>[2x]MSQEQLVAVNELNENLGKVLIKIARDSIANKLGILKINLEDYLSSLNDPI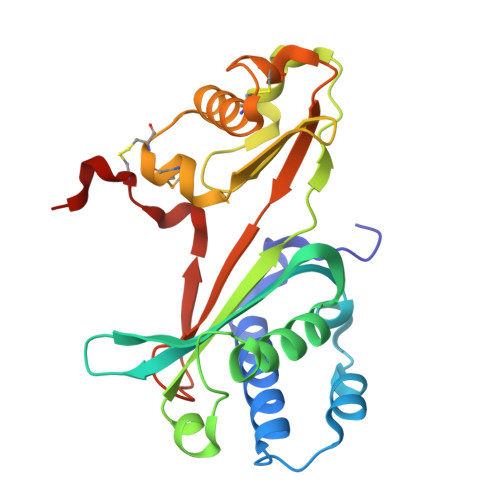LNKKGLAFVTLETYYGNSTSLRGCIGYVEAVAPLKEIVSKAAIAAAFSDPRFPPLSKGEFDNIIIEVTVLTKPQEIDVENRWELPKKIKVGEDGLIVEYGILYSGLLLPQVPMEYCWDEETFLAETCIKAGLEPDCWLNNKVKIKKFQGIIFREEKPKSEKILIIKPSEVKCKKEEISLL(1S,3S,4S)-1,3,4-TRIPHOSPHO-MYO-INOSITOL 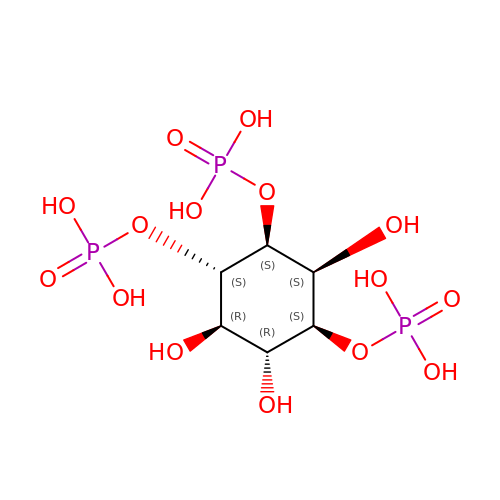| C6 H15 O15 P3 | MMWCIQZXVOZEGG-MLQGYMEPSA-N>MLLAALLAALVARTTLGADVDAVPAPTFPPPAYPYTESWQLTLTTVPSPFVGPADVYHTRPLEDPCGVVALISDPQVDRLLNEAVAHRRPTYRAHVAWYRIADGCAHLLYFIEYADCDPRQVFGRCRRRTTPMWWTPSADYMFPTEDELGLLMVAPGRFNEGQYRRLVSVDGVNILTDFMVALPEGQECPFARVDQHRTYKFGACWSDDSFKRGVDVMRFLTPFYQQPPHREVVNYWYRKNGRTLPRAYAAATPYAIDPARPSAGSPRPRPRPRPRPRPKPEPAPATPAPPDRLPEPATRDHAAGGRPTPRPPRPETPHRPFAPPAVVPSGWPQPAEPFQPRTPAAPGVSRHRSVIVGTGTAMGALLVGVCVYIFFRLRGAKGYRLLGG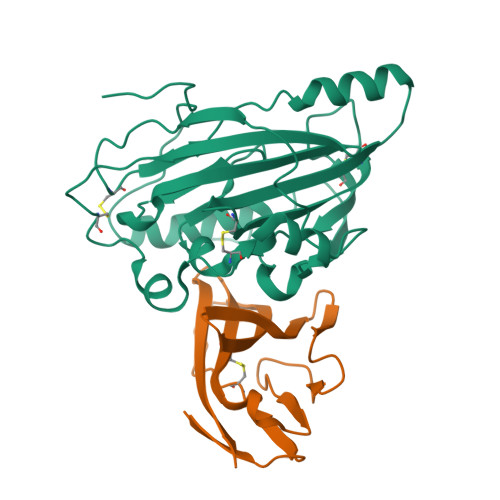PADADELKAQPGP[2x];>DSMYGFIGTDVVLHCSFANPLPGVKITQVTWQKATNGSKQNVAIYNPAMGVSVLAPYRERVEFLRPSFTDGTIRLSRLELEDEGVYICEFATFPAGNRESQLNLTVM[2x]>MGHHHHHHMKAGLNLPAKDRRFKTADVTDTKGVEFEDFCLGRDLLMGIFEKGWEKPSPIQEASIGVALTGQDILARAKNGTGKTGAYCIPVIEKIQPALKAIQAMVIVPTRELALQTSQICVELSKHIQLKVMVTTGGTDLRDDIMRLNGTVHLVIATPGRILDLMEKGVAKMEHCKTLVLDEADKLLSQDFQGILDRLINFLPKERQVMLYSATFPNTVTSFMQKHMHKPY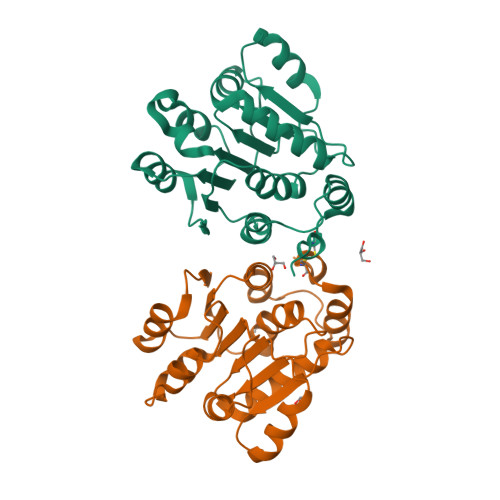EINLME[2x]> STQEQTPQICVVGSGPAGFYTAQHLLKHHSRAHVDIYEKQLVPFGLVRFGVAPDHPEVKNVINTFTQTARSDRCAFYGNVEVGRDVTVQELQDAYHAVVLSYGAEDHQALDIPGEELPGVFSARAFVGWYNGLPENRELAPDLSCDTAVILGQGNVALDVARILLTPPDHLEKTDITEAALGALRQSRVKTVWIVGRRGPLQVAFTIKELREMIQLPGTRPMLDPADFLGLQDRIKEAARPRKRLMELLLRTATEKP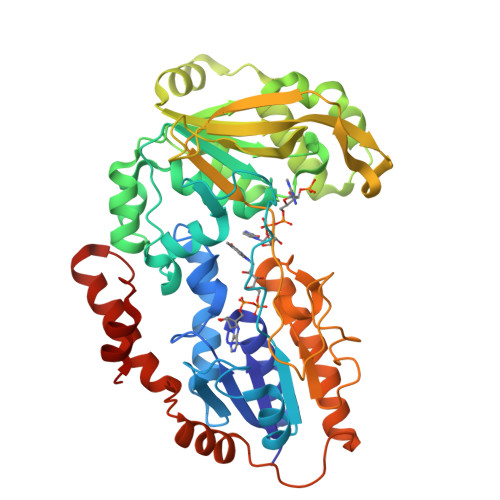GVEEAARRASASRAWGLRFFRSPQQVLPSPDGRRAAGIRLAVTRLEGIGEATRAVPTGDVEDLPCGLVLSSIGYKSRPIDPSVPFDPKLGVVPNMEGRVVDVPGLYCSGWVKRGPTGVITTTMTDSFLTGQILLQDLKAGHLPSGPRPGSAFIKALLDSRGVWPVSFSDWEKLDAEEVSRGQASGKPREKLLDPQEMLRLLGH> TIEERVKKIIGEQLGVKQEEVTNNASFVEDLGADSLDTVELVMALEEEFDTEIPDEEAEKITTVQAAID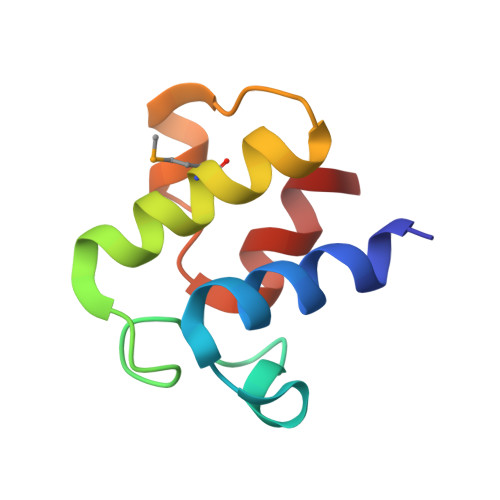YIN1-{(1S)-1-[4-(3-amino-1H-indazol-6-yl)-5-chloro-1H-imidazol-2-yl]-2-phenylethyl}-3-[2-(aminomethyl)-5-chlorobenzyl]urea 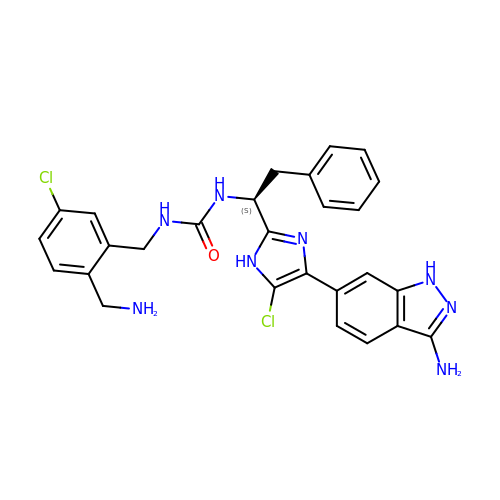| C27 H26 Cl2 N8 O | PKKLAAQPYSEUAW-QFIPXVFZSA-N>[4x]SDRLNSGHQLD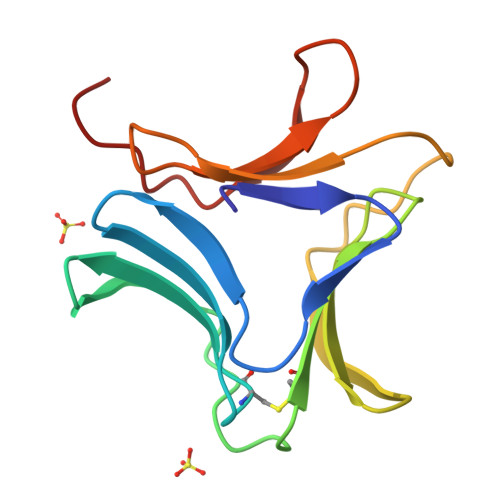TGGSLAEGGYLFIIQNDCNLVLYDNNRAVWASGTNGKASGCVLKMQNDGNLVIYSGSRAIWASNTNRQNGNYYLILQRDRNVVIYDNSNNAIWATHTNVGN4N-MALONYL-CYSTEINYL-2,4-DIAMINOBUTYRATE DISULFIDE | C20 H32 N6 O12 S2 | 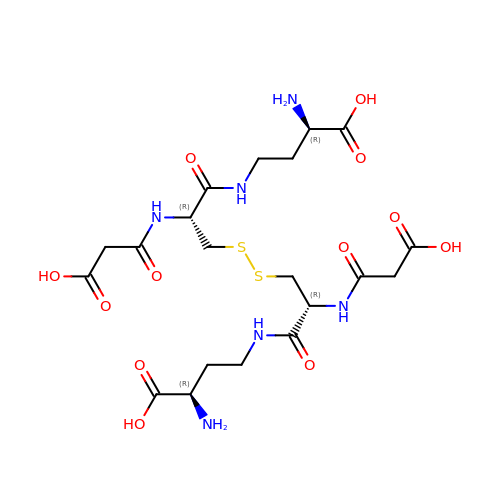MRZMTLNHPCSZCE-NNYUYHANSA-N>[2x]LGNFSQACYNSAIQGSVLTSTCIRTNGGYNTSSIDLNSVIENV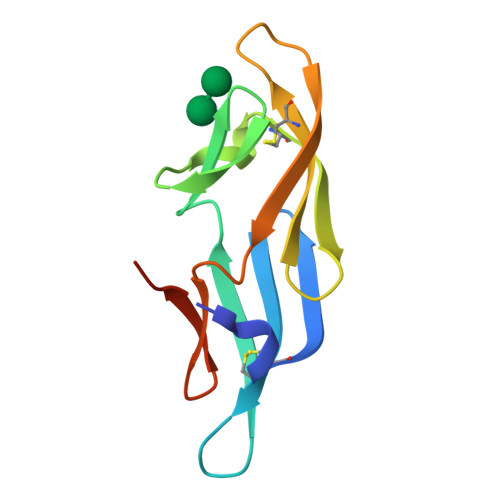DGSLKWQGSNFIETCRNTQLAGSSELAAECKTRAQQFVSTKINLDDHIAAIDGTLKYELEHHHHHH> MPFTIDSARGIFPETLTADSVPATIARFNQLSAEDQLALIWFAYLEMGKTITIAAPGAANMVFAENTLNELKQMSFQEQTQVMCDLANRADTPICRTYAIWSVNIKLGFWYRLAEWMEQGIVAPIPQGYRLSANAAAVLQAIRELDAGQQITVLRNSVVDMGYDPSKLGSYTKVSEPVAPPKEMAKRTPVTIEGIDNPTILSYMDNLNANDFDALIELFTPDGALQPPFQKPIAGKEAVYRFFREDCQNLKLIPQRGVSEAVEDGYTQIKVTGTVQTPWFGASVGMNMAWRFLLTPENKIFFVAIDLLASPKELL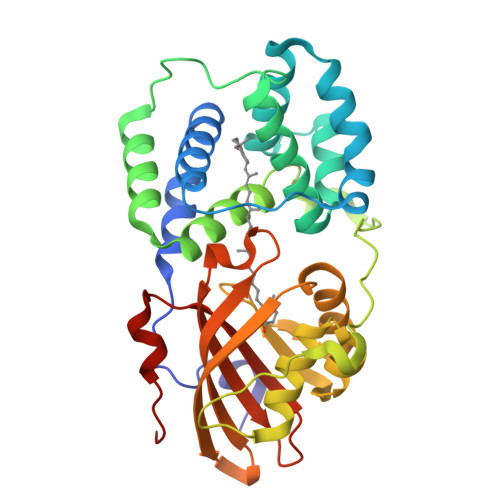NLVRHHHHHHH>GPGHMELRSKREKASRVHEVIIFNELGEICAAVHMRNSSMGSQKPQVSPCCN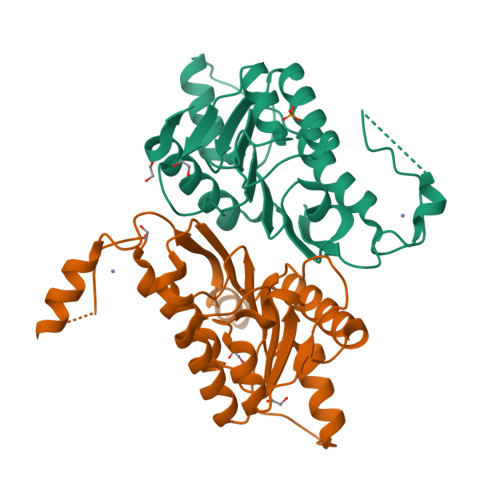THCSLRNVAKIVEQIDRAVYSIDLAIYTFTSLFLADSIKRALQRGVIIRIISDGEMVYSKGSQISMLAQLGVPVRVPITTNLMHNKFCIIDGFERVEEIRLLRKLKFMRPCYSIVISGSVNWTALGLGGNWENCIITADDKLTATFQAEFQRMWRAFAKTEGSQIQLK[2x]>[2x]TNPVLDVDGNELQR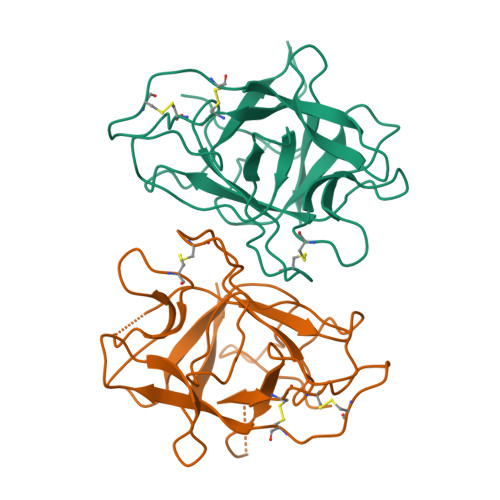GQLYYATSVMRPGGGLTLAAPKGSCPLNVAQAPFDEYSGRPLAFFPENADDDTVQEGSTLYIMFPEPTRCPQSTVWTFDREAGFVTTGGTTSKAIGPHNSRFAIRKAGDASSQPRDYQIEVCPCSTGVERPSCRMGCLGTLGLAEGGKNVLLNINNESPHTIRFVKVKEG>[5x]SN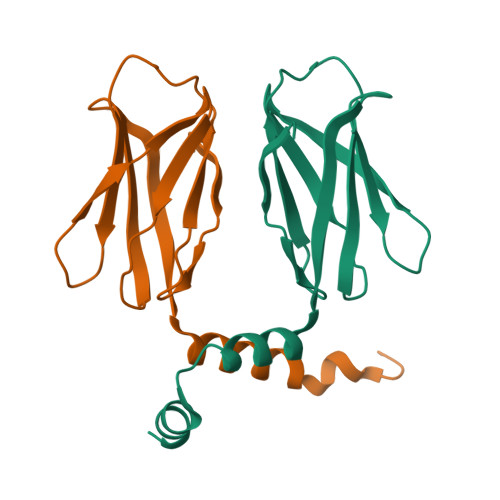AMVVQPDRIRCGAETTVYVIVRCKLDDRVATEAEFSPEDSPSVRMEAKVENEYTISVKAPNLSSGNVSLKIYSGDLVVCETVISYYTDMEEIGNLLSNAANPVEFMCQAFK Growth/differentiation factors 8 and 11 (GDF8/myostatin and GDF11/BMP11, respectively) are two closely related members of the activin/inhibin subclass that share ~90% sequence identity in their mature, C-terminal signaling domains and ~52% identity in their N-terminal prodomains. Similar to other TGFβ ligands, GDF8 and GDF11 are disulfide-linked dimers that are initially synthesized as precursors, which are cleaved by furin-like proteases to separate the N-terminal prodomain from the C-terminal mature domain. The ligand dimer elicits signal transduction by symmetrically binding two type II and two type I transmembrane serine/threonine kinase receptors. Similar to other ligands in the activin/inhibin subclass, GDF8 and GDF11 predominantly signal through the type II receptors, activin receptor kinase IIA (ActRIIA; ACVR2A) and ActRIIB (ACVR2B) and the type I receptors, activin-like receptor kinase 4 (ALK4; ACVR1B) and ALK5 (TβRI).

We resolved the structure of apo-GDF8 to 2.25 Å and the apo-GDF11 structure to 1.90 Å using X-ray crystallography, thus allowing a direct comparison to the recently published apo-GDF11 structure (middle). Unexpectedly, resolution of the apo-GDF8 structure revealed a unique conformation such that the fingertips of each monomer are positioned proximally in a “closed” conformation compared to the classical distal positioning or “open” conformation observed for many ligands, including structures of FS-bound GDF8 (top). While the structure of apo-GDF8 adopted an unexpected “closed” conformation, a similar conformation has been observed for activin A when in complex with ActRIIB. In both cases, the wrist region is disordered and not resolved in the crystal structure. The extreme “closed” conformation of GDF8 is not entirely unprecedented, as one structure of activin A in complex with ActRIIB showed a similar “closed” configuration. Interestingly and despite the high sequence identity, nearly identical crystallization conditions resulted in two distinct conformations. Although these conformations may be a result of the crystallization process, it supports the idea that GDF8 and GDF11 are flexible enough to be trapped in alternate states. Taken together, crystallization of both GDF8 and GDF11 in their apo states reveals intrinsic structural flexibility in these ligands.

>[2x]DFGLDCDEHSTESRCCRYPLTVDFEAFGWDWIIAPKRYKANYCSGECEFVFLQKYPHTHLVHQANPRGSAGPCCTPTKMSPINMLYFNGKEQIIYGKIPAMVVDRCGCS>GAM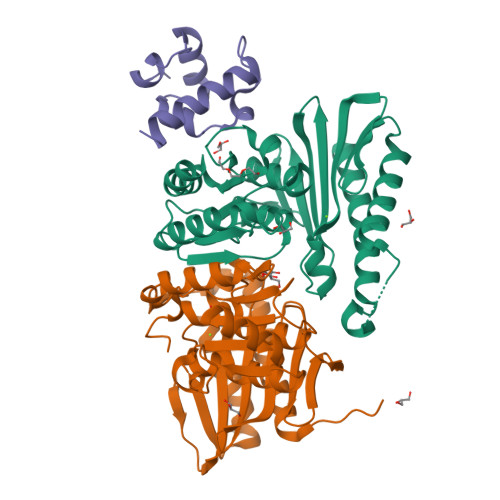AMHPMLNIAVRAARKAGNLIAKNYETPDAVEASQKGSNDFVTNVDKAAEAVIIDTIRKSYPQHTIITEESGELEGTDQDVQWVIDPLDGTTNFIKRLPHFAVSIAVRIKGRTEVAVVYDPMRNELFTATRGQGAQLNGYRLRGSTARDLDGTILATGFPFKAKQYATTYINIVGKLFNECADFRRTGSAALDLAYVAAGRVDGFFEIGLRPWDFAAGELLVREAGGIVSDFTGGHNYMLTGNIVAGNPRVVKAMLANMRDELSDALKR[2x];> GAMDNKPADDLLNLEGVDRDLAFKLAARGVCTLEDLAEQGIDDLADIEGLTDEKAGALIMAARNICWFGDEA UdgX excises uracil from uracil-containing DNA to concurrently form a covalent bond with the resulting AP-DNA. Structurally, UdgX is highly similar to family-4 UDGs (F4-UDGs). However, UdgX is unique in possessing a flexible R-loop (105KRRIH109). Our earlier studies allowed us to propose a reaction mechanism of UdgX, which involves the formation of a covalent bond between H109 of UdgX with the C1′ position of the target deoxyribose sugar concurrently with the uracil excision from this site in DNA.

Based on our previous structural analysis, we had proposed that E52 participates in a catalytic dyad with H109 to activate it for a nucleophilic attack onto C1′ position of the target the deoxyribose sugar cation. Further, in the structure of H109S mutant, a water molecule was appropriately located near S109 for activation by E52 (26). To further validate the role of E52, we combined the H109S mutation (where a water molecule is allowed to locate in place of His ring) with the E52N mutation and assessed its effect on the uracil excision activity. Expectedly, the uracil excision activity of the double mutant (H109S/E52N) was lowered compared to the H109S mutant. The Kcat of the double mutant (H109S/E52N) decreased by ∼10-fold as compared to the H109S. The Km of the double mutant increased by ∼7-fold, resulting in an overall reduction of ∼75-fold in Kcat/Km. Consistent with these observations, the distance of 4.71 Å between OG of S109 and OE2 of E52 in the H109S mutant increased to 5.71 Å between OG of S109 and ND2 of N52 in the H109S/E52N mutant. The E52Q, E52N and E52A mutants reveal that E52 forms a catalytic dyad with H109 to enhance its nucleophilicity.

> MAGAQDFVPHTADLAELAAAAGECRGCGLYRDATQAVFGAGGRSARIMMIGNQPGDKEDLAGLPFVGPAGRLLDRALEAADIDRDALYVTNAVKHFKFTRAAGGKRRISKTPSRTEVVACRPWLIAEMTSVEPDVVVLLGATAAKALLGNDFRVTQHRGEVLHVDDVPGDPALVATVHPSSLLRGPKEERESAFAGLVDDLRVAADVR> M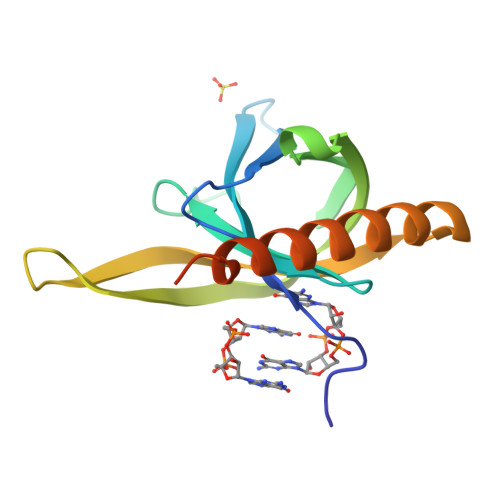QRRRYFRISAPLHPPYFCQTKLADNSTLRFRLYDLSLGGMGALLETAKPAELQEGMRFAQIEVNMGQWGVFHFDAQLISISERKVIDGKNETITTPRLSFRFLNVSPTVERQLQRIIFSLEREAREKADKVRDKLAAALEHHHHHH>HHHHHHASENLYFQGAMASEKHFKYVILGGGVAAGYAAREFAKQGVKPGELAIISKEAVAPYERPALSKGYLFPQNAARLPGFHVCVGSGGERLLPEWYSEKGIELILSTEIVKADLASKTLTSAVGATFTYEILIIATGSSVIKLSDFGTQGADSNNILYLREVDDADKLVAAIQAKKGGKAVIVGGGYIGLELSAALKINDFDVTMVFPEPWCMPRLFTADIAAFYESYYTNKGVKIVKGTVAVGFDADANGDVTAVNLKNGSVLEADIVVVGVG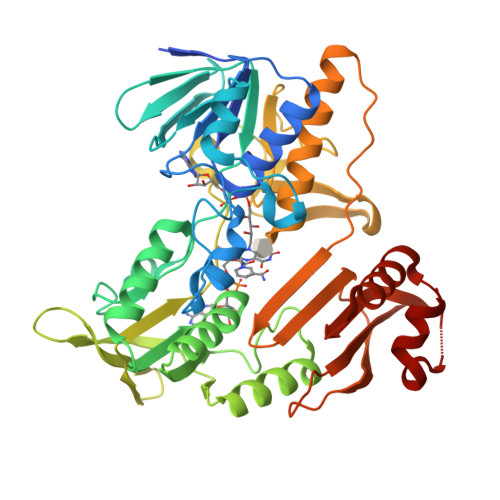GRPLTTLFKGQVAEEKGGIKTDAFFETSVPGVYAVGDVATFPMKMYNELRRVEHVDHARKSAEQAVKAIKGKESGESVVEYDYLPYFFSRSFDLGWQFYGDNVGDTILFGDSDPTSAKPKFGSYWIKDGKVLGAFLEGGSPDENKAIAKVAKTQPPVANIEELKKEGLQFASKI[2x]> AKMMQREITKTTVNVAKMVMVDGEVQVEQLPSETFVGNLTMEQAQWRMKRKYKGEPVQVVSVEPNTEVYELP

The genome-organizing protein p6 of Bacillus subtilis bacteriophage φ29 plays an essential role in viral development by activating the initiation of DNA replication and participating in the early-to-late transcriptional switch. These activities require the formation of a nucleoprotein complex in which the DNA adopts a right-handed superhelix wrapping around a multimeric p6 scaffold, restraining positive supercoiling and compacting the viral genome. Additionally, p6 forms dimers that bind to DNA every 24 nucleotides and interact with the viral DNA through the minor groove. In this work, we have shown that protein p6 showcases a remarkable evolutionary design that encompasses a folded core as its foundation, upon which, two structural regions play crucial roles in dimerization and oligomerization.

In a first attempt, we removed the final 31 residues (encompassing the α2 together with the C-terminal disordered acidic tail) with the aim of generating a minimal truncated protein fragment suitable for crystallization. After purifying the resulting variant, denoted as p6CΔ31, we efficiently obtained well-diffracting crystals that permitted its structural determination at ∼1.6 Å resolution (experimental electron density is shown in Supplementary Figure S2E). A comparison between the experimental p6CΔ31 structure and the AF2 prediction revealed nearly identical backbone structures, with a rmsd of only 0.664 Å across 53 pruned atom pairs. The folded core of p6CΔ31 assembles into a concave four-stranded antiparallel β-sheet (β1–β4). The central feature of this fold comprises the β1 strand interacting in an antiparallel orientation with the adjacent β2 and β4 at one side, and with β3 on the other. Furthermore, a 12 residues-long α-helix (α1) bridges β3 and β4 strands and packs against β1, β3 and β4. This spatial arrangement builds up a compact and well-ordered core facilitated by the burial of numerous hydrophobic residues (V13, V15, L30, F35, L39, M41, A44, M48, Y52, V57, V59 and V62). In the crystallographic structure of p6CΔ31, residues 1–8 and 68–72, which would extend β1 and β4 strands, respectively, are not visible despite their inclusion in the construct's sequence. This likely results from the absence of stabilizing interactions provided by the α2 within this region when the protein is in a dimeric state (see next section). Further deletion involving the α2 helix (p6CΔ31) completely abolished dimerization (not shown).>MATEQIQHIAIVGCVHGKYREMYRQLSEYEKSTGKEISFVICTGDMQTLRYEADLVYLKVPPKYKQMGDFHLYYEGKEKAPYLTLFIGGNHESSNVLLHLYNGGFVCFNMYYLGVCSCININGLRIVGVSGIYKSFDEKKPYTYPPSPNDVVSLFHTRNYVIQMLSNLSQSSQIDISLSHDWPQGIVMKGNYKQLYRFQPGFKKDGASLGSPINKVILNTLKPKYWISGHMHCEYHAEEGPTHFIALGKIGYKNAISYLDLPLKQKTDLEYDKDWVCNLIMTWPAFSNKAQFPDLSYSISELLSKRTKELD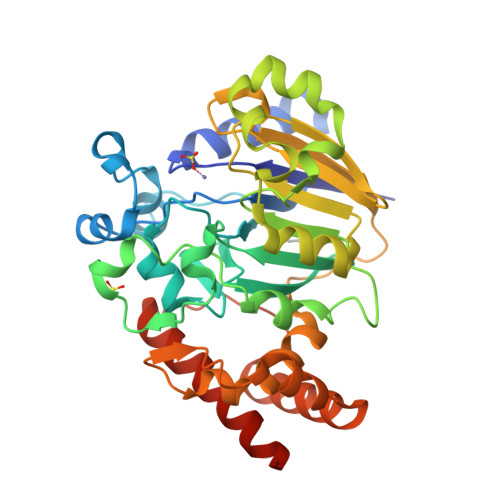KKIIELWEKYIGLKIIYDSDTFDIQFTSRRFYIEKIYNELNINHHHHHH[5x]> GPHMLEMPKEKYEPPDPRRMYTIMSSEEAANGKKSHWAELEISGKVRSLSASLWSLTHLTALHLSDNSLSRIPSDIAKLHNLVYLDLSSNKIRSLPAELGNMVSLRELHLNNNLLRVLPFELGKLFQLQTLGLKGNPLTQDILNLYQEPDGTRRLLNYLLDNLSGTAKRITTEQPPPRSWIMLQEPDRTRPTALFSVMCYNVLCDKYATRQLYGYCPSWALNWDYRKKAIIQEILSCNADIVSLQEVETEQYYSFFLVELK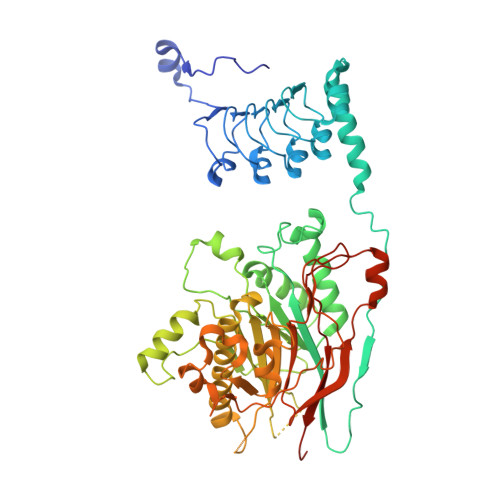ERGYNGFFSPKSRARTMSEQERKHVDGCAIFFKTEKFTLVQKHTVEFNQLAMANSEGSEAMLNRVMTKDNIGVAVLLELRKESIEMPSGKPHLGTEKQLILVANAHMHWDPEYSDVKLVQTMMFLSEVKNIIDKASRNLKSSVLGEFGTIPLVLCADLNSLPDSGVVEYLSTGGVETNHKDFKELRYNESLTNFSCHGKNGTTNGRITHGFKLQSAYESGLMPYTNYTFDFKGIIDYIFYSKPQLNTLGILGPLDHHWLVENNISGCPHPLIPSDHFSLFAQLELLLPFLPQVNGIHLPGRR> MSNFIFGRYLPLDSVVHRL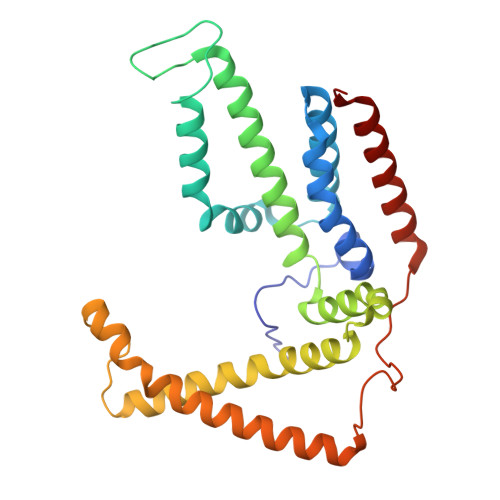DPRAKLMLSFCYIIVVFLANNIWSYAILIAFTVGAILSSKISLGFFLKGIRPLLWLIVFTVVLQLLFSPAGGHTYFHWAFINVTQDGLINAGYIFVRFLLIIMMSTLLTLSTQPLDIATGLASLMKPLRWVKVPVDTLAMMLSIALRFVPTLMDEATKIMNAQRARGVDFGEGGLFKQAKSLIPLMVPLFMSAFNRAEDLSTAMEARGYQDSEHRSQYRILTWQRRDTVTWLLFLLGFVAILIFRHW>ADDYLQHSIVPTMHYQDSLPRLPIPKLEDTMKRYLNAQKPLLDDSQFRRTEALCKNFETGVGKELHAHLLAQDKQNKHTSYISGPWFDMYLTARDSIVLNFNPFMAFNPDPKSEYNDQLTRATNLTVSAVRFLKTLQAGLLEPEV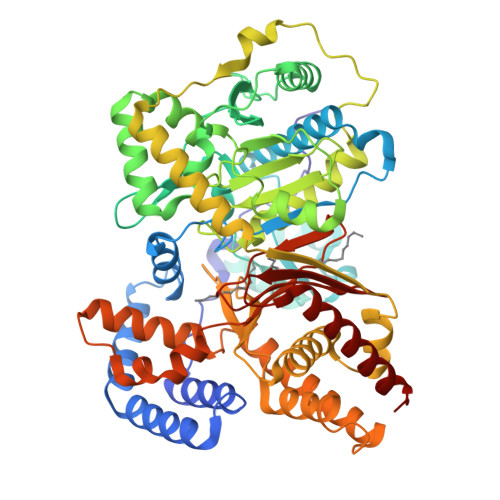FHLNPSKSDTDAFKRLIRFVPPSLSWYGAYLVNAYPLDMSQYFRLFNSTRIPRPNRDELFTDTKARHLLVLRKGHFYVFDVLDQDGNIVNPLEIQAHLKYILSDSSPVPEFPVAYLTSENRDVWAELRQKLIFDGNEETLKKVDSAVFCLCLDDFPMKDLIHLSHTMLHGDGTNRWFDKSFNLIVAEDGTAAVHFEHSWGDGVAVLRFFNEVFRDSTQTPAITPQSQPAATNSSASVETLSFNLSGALKAGITAAKEKFDTTVKTLSIDSIQFQRGGKEFLKKKQLSPDAVAQLAFQMAFLRQYGQTVATYESCSTAAFKHGRTETIRPASIFTKRCSEAFVRDPSKHSVGELQHMMAECSKYHGQLTKEATMGQGFDRHLYALRYLATARGLNLPELYLDPAYQQMNHNILSTSTLNSPAVSLGGFAPVVPDGFGIAYAVHDDWIGCNVSSYSGRNAREFLHCVQKCLEDIFDALEGKAI[2x]> MIEPPVIDPAAVPPDETGPDNPMEQRRVCAAPTVYPDSNFADRPWASDYLRLTEAHKFATGAGITVAVIDTGVNGSPRVPAEPGGDFVDAAGNGMSDCDAHGTLTASVIAGRGAPTDGFIGVAPDARILSLRHTSAAFQPVGART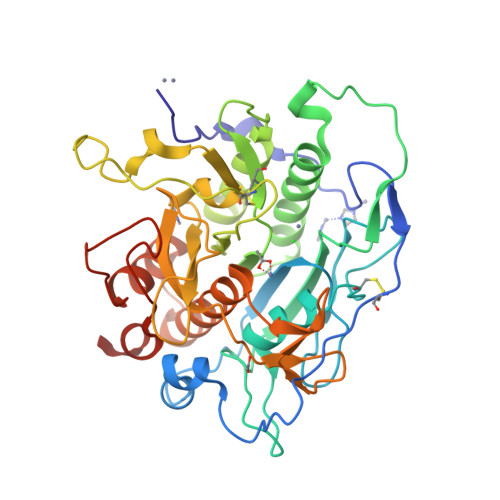DPNNPNTTQTAGSLRSLARAIVHAANLGAQVINISEAACYKVTRPIDETGVGAAVNYAVHVKNAVVIAAAGNTGQDCTQNPPPDPAVPSDPRGWQQVQTIVSPAWYSPLVLTVGGIGPTGQPSNFSMSGPWVGAAAPAENITALGYGGEPVNALQGQDGLVPVAGTSFAAAYVSGLAALIRQRYPDLTPAQVINRITATARHPGGGVDNYVGAGVIDPVAALTWDVENLYFQ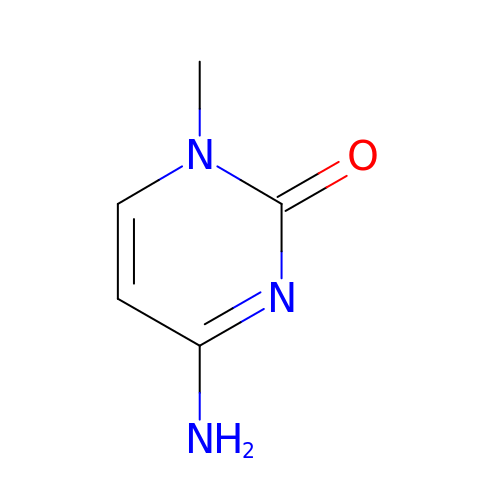1-METHYLCYTOSINE | C5 H7 N3 O | HWPZZUQOWRWFDB-UHFFFAOYSA-N> GAMAVKVARPCRKIEKWTYLELKGSKANEGVPQAMTAFAEFLNRTGIPINPRFSPGMSMSVPGSEKEFFAKVKELMSSHQFVVVLLPRKDVAIYNMVKRAADITFGVHTVCCVAEKFLSTKGQLGYF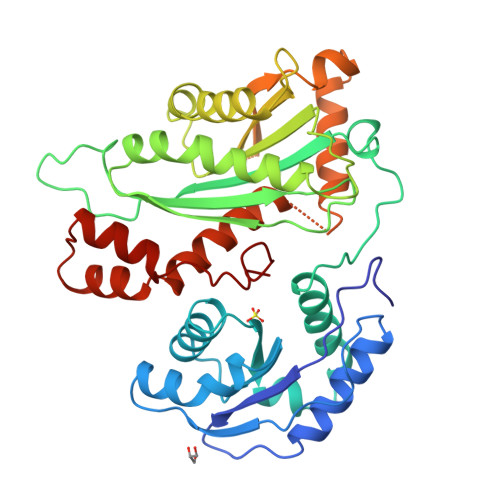ANVGLKVNLKFGGTNHNIKTPIPLLAKGKTMVVGYDVTHPTNLAAGQSPASAPSIVGLVSTIDQHLGQWPAMVWNNPHGQESMTEQFTDKFKTRLELWRSNPANNRSLPENILIFRDGVSEGQFQMVIKDELPLVRAACKLVYPAGKLPRITLIVSVKRHQTRFFPTDPKHIHFKSKSPKEGTVVDRGVTNVRYWDFFLQAHASLQGTARSAHYTVLVDEIFRADYGNKAADTLEQLTHDMCYLFGRATKAVSICPPAYYADLVCDRARIHQKELFDALDENDSVKTDDFARWGNSGAVHPNLRNSMYYI>[2x]MALSTATKAATDALAANRAPTSVNAQEVHRWLQSFNWDFKNNRTKYATKYKMANETKEQFKLIAKEYARMEAVKDERQFGSLQDALTRLNAGVRVHPKWNETMKVVSNFLEVGEYNAIAATGMLWDSAQAAEQKNGYLAQVLDEIRHTHQCAYVNYYFAKNGQDPAGHNDARRTRTIGPLWKGMKRVFSDGFISGDAVECSLNLQLVGEACFTNPLIVAVTEWAAANGDEITPTVFLSIETDELRHMANGYQTVVSIANDPASAKYLNTDLNNAFWTQQKYFTPVLGMLFEYGSKFKVEPWVKTWD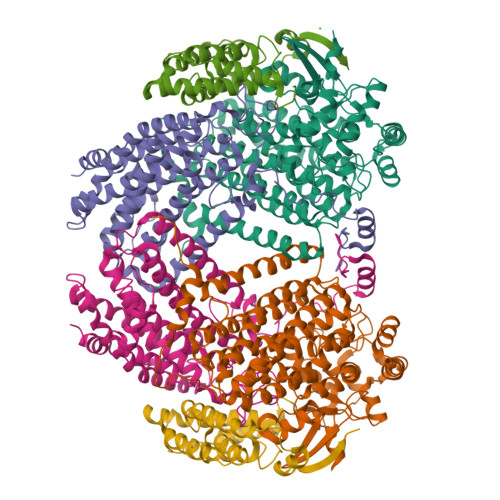RWVYEDWGGIWIGRLGKYGVESPRSLKDAKQDAYWAHHDLYLLAYALWPTGFFRLALPDQEEMEWFEANYPGWYDHYGKIYEEWRARGCEDPSSGFIPLMWFIENNHPIYIDRVSQVPFCPSLAKGASTLRVHEYNGEMHTFSDQWGERMWLAEPERYECQNIFEQYEGRELSEVIAELHGLRSDGKTLIAQPHVRGDKLWTLDDIKRLNCVFKNPVKAFN;>[2x]SMLGERRRGLTDPEMAEVILKALPEAPLDGNNKMGYFVTPRWKRLTEYEALTVYAQPNADWIAGGLDWGDWTQKFHGGRPSWGNETTELRTVDWFKHRDPLRRWHAPYVKDKAEEWRYTDRFLQGYSADGQIRAMNPTWRDEFINRYWGAFLFNEYGLFNAHSQGAREALSDVTRVSLAFWGFDKIDIAQMIQLERGFLAKIVPGFDESTAVPKAEWTNGEVYKSARLAVEGLWQEVFDWNESAFSVHAVYDALFGQFVRREFFQRLAPRFGDNLTPFFINQAQTYFQIAKQGVQDLYYNCLGDDPEFSDYNRTVMRNWTGKWLEPTIAALRDFMGLFAKLPAGTTDKEEITASLYRVVDDWIEDYASRIDFKADRDQIVKAVLAGLK;>AKLGIHSNDTRDAWVNKIAQLNTLEKAAEMLKQFRMDHTTPFRNSYELDNDYLWIEAKLEEKVAVLKARAFNEVDFRHKTAFGEDAKSVLDGTVAKMNAAKDKWEAEKIHIGFRQAYKPPIMPVNYFLDGERQLGTRLMELRNLNYYDTPLEELRKQRGVRVVHLQSPH[2x]In this work, we exhaustively probe the ability of all 36 immobile HJ sequences to form DNA crystals in two different designed systems. Three separate self-assembling DNA crystal systems are described in this report: the “4 × 5” and “4 × 6” designs (collectively referred to as the 4 × N systems), and a third construct with a “scrambled” sequence variant of the 4 × 6 lattices. Self-assembly was mediated by three constituent oligonucleotides: (S1) containing four sequence repeats of either 5 or 6 bases; (S2) composed of 21 bases containing complementary regions to both (S1); and (S3) which forms the second junction crossover. The HJ serves as the fundamental component at the core of each unit, and the ultimate assembly of the full lattice is facilitated by the complementary 2-base sticky ends that tail each duplex.

To investigate this possibility, we designed “scrambled” sequences with targeted base substitutions, while maintaining GC content, along each “stem”. Contrary to the buffer preference observed with the native P32 crystals, the scrambled systems exhibited an exclusive preference towards low salt buffers, much like the native R3 crystals. Remarkably, only J1 and J2 retained the P32 symmetry, with all others yielding an R3 lattice. There appeared to be only a marginal difference in the average cell lengths in the R3 scramble crystals (a = b = 113.04 c = 51.10) relative to the native 4 × 6 sequences: the a, b axis trended ~2 Å shorter and c ~1.3 Å longer, whereas in the J1 and J2 cases, the crystals were in good agreement with the original 4 × 6 motif. The average angles of the R3 and P32 crystals were 61.00° (σ = 1.21) and 58.05° (σ = 1.39), respectively. Another major observation is the importance of stem region sequences outside the HJ, given that this sequence can control crystal symmetry and lattice architecture, and improve resolution in non-obvious ways.

> GAACGACATTGA;> CGAGGACTC;> TCATCG;> TCGAGTCCATGTCGT> GPLGSPNSEEEASVSVWDEEEDGATFTVTSRQYRPLDPLAPLPPPRSSRRLRAGTLEALVRHLLDARTAGADMMFTPALLATHRAFTSTPALFGLVADRLEALESYPPGELERTTGVAISVLSTWLASHPEDFGSEVKGQLDRLESFLLRTGYAAREGVVGGSADLIRNLRARVDPRAPDLPKPLALPGDSPADPTDVLVFLADHLAEQLTLLDAELFLNLIPSQCLGGLWGHRDRPGHSHLCPSVRATVTQFNKVAGAVVSSVLGATSIGEGPREVTVRPLRPPQRARLLEKWIRVAEECRLLRNFSSVYAVVSALQSSPIHRLRAAWGETTRDSLRVFSSLCQIFSEEDNYSQSRELLTQEVKPQPPVEPHSKKAPRSGFRGGGVVPYLGTFLKDLV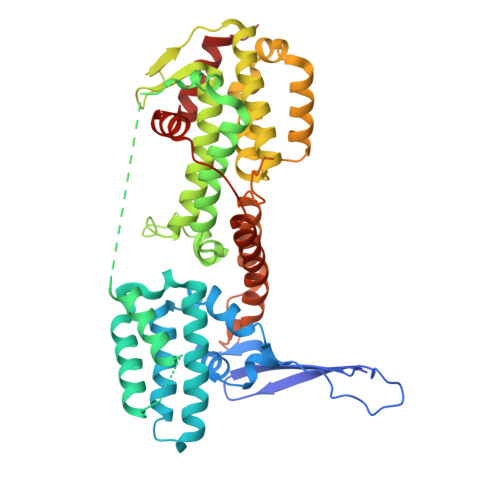MLDAASKDELENGYINFDKRRKEFAILSELLRLQKECRGYDLRPNSDIQQWLQGLQPLTEAQSHRVSCEVEPPG>[3x]SRCTHLENRDFVTGTQGTTRVTLVLELGGCVTITAEGKPSMDVWLDAIYQENPAKTREYCLHAKLSDTKVAARCPTMGPATLTEEHQGGTVCKRDQSDRGWGNHCGLFGKGSIVACVKAACEAKKKATGHVYDANKIVYTVKVEPHTGDYVAANETHSGRKTASFTVSSEKTILTMGEYGDVSLLCRVASGVDLAQTVILELDKTVEHLPTAWQVHRDWFNDLALPWKHEGAQNWNNAERLVEFGAPHAVKMDVYNLGDQTGVLLKALAGVPVAHIEGTKYHLKSGHVTCEVGLEKLKMKGLTYTMCDKTKFTWKRAPTDSGHDTVVMEVTFSGTKPCRIPVRAVAHGSPDVNVAMLITPNPTIENNGGGFIEMQLPPGDNIIYVGELSHQWFQKGSSIGRVFQKTKKGIERLTVIGEHAWDFGSAGGFMTSIGRAMHTVLGGAFNTLLGGVGFLPKILLGVAMAWLGLNMRNPTLSMGFLLSGGLVLAMTLGVGA;>SVLIPSHAQGELTGRGHKWLEGDSLRTHLTRVEGWVWKNKLLALAMVTVVWLTLESVVTRVAVLVVLLCLAPVYA[3x]

The E protein is a class II fusion protein and the largest of the structural proteins. It is the main protein responsible for receptor binding and fusion, as well as the major target for neutralizing antibodies. The prM protein is a precursor that is cleaved by the host cell protease furin into mature M protein and a pr peptide.

We thoroughly characterized a chimeric virus containing the prM and ectodomain of E (ecto-E) proteins of TBEV in a LGTV genetic background. We determined the structures of LGTV and chimeric LGTVT:prME using cryogenic electron microscopy (cryo-EM) and three-dimensional image reconstruction. There are three occurrences of M in the asymmetric unit. In one of these three, we modeled two alternative conformations for residues 25–74 of LGTVT:prME. One conformation is identical to LGTV and TBEV, maintaining the pi-stacking interactions between M residues Trp37 at the raft interfaces, as well as the salt bridges between Lys40 and Glu33 of the respective chains, whereas the alternative conformation disrupts these tight interactions. The new models included two extra residues in the C-terminus of the E protein (residues 495 and 496), and the LGTVT:prME model has one more residue in the C-terminus of the M protein (residue 75). The observed attenuation might also be due to sub-optimal interactions between the prM protein from TBEV and the C protein or transmembrane domain of the E protein of LGTV.> SNAHGFHMPAEWEPHSQCWIGWPERADNWRDGAVHAQLVFTRVAAAISRFEKVTVCASSAQWENARNQLPDHVRVVEISSNDSWFRDIGPTFVVRRETSKSDDAEHRIAGIDWTFNSWGGLEDGCYCDWSLDSLVKKKILDVERIPRFSHSMVLEGGSIHVDGEGTCITTEECLLNKNRNPHLSKSQIEDELKAYLGVRKVIWLPRGLYGDDDTNGHVDNMCCFVRPGAVLLSWTDDKTDPQYERSEEAYSLFSSVTDANGRKFEVIKLHVPGPLYMTEKEAAGVFQDDGAKPRLPGTRLAASYVNFYIANGAIIAPQFGDKKWDDEAIRVLSKTFPHHEVVGIEGSREIVLSGGNIHCITQQQPAI

Herein, we describe the structural characterization of AIH from Medicago truncatula (MtAIH), the model legume plant. The enzyme is responsible for the second step of the AGM pathway of PUT biosynthesis, that is the hydrolytic conversion of AGM to N-carbamoylputrescine (NCP) with the release of ammonia. AIH belongs to one of the seven types of guanidine-modifying enzymes (GMEs). It is a member of the pentein superfamily that is characterized by the propeller-like arrangement of five repeated motifs that form a narrow channel with a central, negatively charged core. The monomer of MtAIH is no different in this matter, i.e., five motif repeats (I–V) are arranged around fivefold pseudosymmetry axis that is aligned with the catalytic tunnel in the core of the protein.

In this work, we present the high-resolution crystal structure of non-liganded MtAIH and the structure with the reaction product analog—6-aminohexanamide (AHX). The envelope with twofold symmetry restraints and ab initio electron density map that was calculated with no information about the molecule symmetry clearly correspond to the MtAIH dimer in the crystal lattice where two subunits are related by twofold symmetry. It is worth to note that both crystal structures, MtAIH and MtAIH-AHX, present different crystallographic symmetry with one and four chains in the asymmetric unit, respectively. In the case of the unliganded structure, the dimer is created by a crystallographic twofold axis, while in the MtAIH-AHX complex, there are two almost identical dimers in the asymmetric unit. The close vicinity of the MtAIH active site is surrounded by two very flexible regions built mostly by long loops. One is the gate-keeping loop covering the active site (residues 291–314), which is a linker between repeat IV and V. The other concerns the fragment 122–136 which belongs to the repeat II, where α4 is located. The gate-keeping loop is very variable in plant AIHs except for Arg301 and Arg306. Both regions are disordered in the non-liganded MtAIH structure, more precisely fragments between Glu129-Cys134 and Pro300-Tyr-293 were excluded from the structure due to the lack of electron density maps that would show their conformation. However, in both MtAIH crystal forms, this interface area between two subunits is preserved and, taking it together with SAXS and MALS results, it is, in fact, responsible for the formation of MtAIH dimers.> MNDRADFVVPDITTRKNVGLSHDANDFTLPQP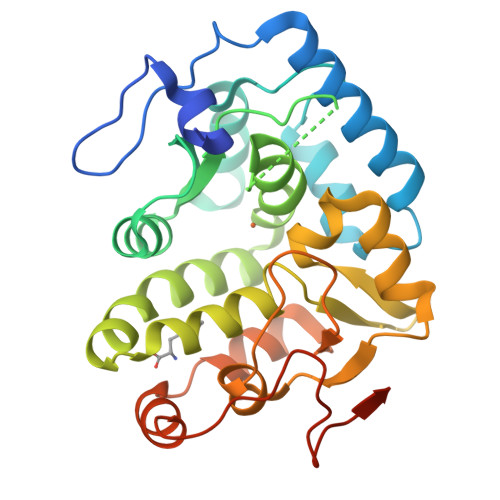LDRYSAEDHATWATLYQRQCKLLPGRACDEFLEGLERLEVDADRVPDFNKLNEKLMAATGWKIVAVPGLIPDDVFFEHLANRRFPVTWWLREPHQLDYLQEPDVFHDLFGHVPLLINPVFADYLEAYGKGGVKAKALGALPMLARLYWYTVEFGLINTPAGMRIYGAGILSSKSESIYCLDSASPNRVGFDLMRIMNTRYRIDTFQKTYFVIDSFKQLFDATAPDFAPLYLQLADAQPWGAGDIAPDDLVLNAGDHQGWADTEDV> AAAAAAAAAAAAAAAAAAAAAAAAAAAAAAAAAAAAAAAA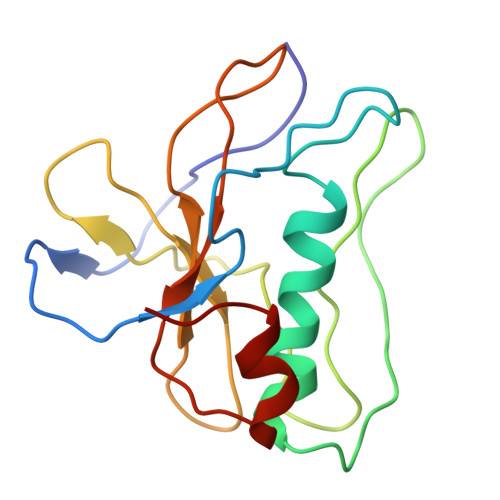AAAAAAAAAAAAAAAAAAAAAAAAAAAAAAAAAAAAAAAAAAAAAAAAAAAAAAAAAAAAAAAAAAAAAAAAAAAAAAAAAAAAAAAAAAAAAAAAAAAAAAAAAAAAAAAA> MENTENSVDSKSIKNLEPKIIHGSESMDSGISLDNSYKMDYPEMGLCIIINNKNFHKSTGMTSRSGTDVDAANLRETFRNLKYEVRNKNDLTREEIVELMRDVSKEDHSKRSSFVCVLLSHGEEGIIFGTNGPVDLAKIT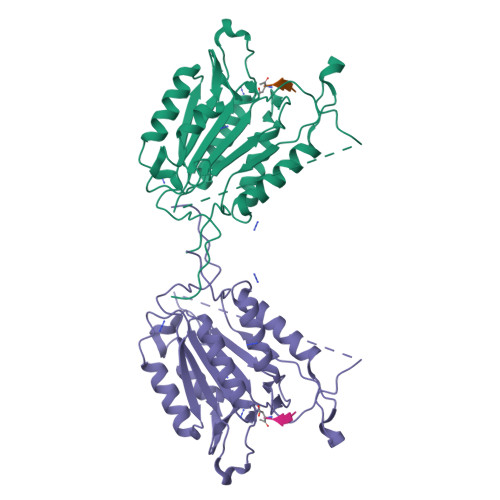NFFRGDRCRSLTGKPKLFIIQACRGTELDCGIETDSGVDDDMACHKIPVEADFLYAYSTAPGYYSWRNSKDGSWFIQSLCAMLKQYADKLEFMHILTRVNRKVATEFESFSFDATFHAKKQIPCIVSMLTKELYFYHHH>GNVGKISLDQIDLLSTKSFPPCMRQLHKALRENHHLRHGGRMQYGLFLKGIGLTLEQALQFWKQEFIKGKMDPDKFDKGYSYNIRHSFGKEGKRTDYTPFSCLKIILSN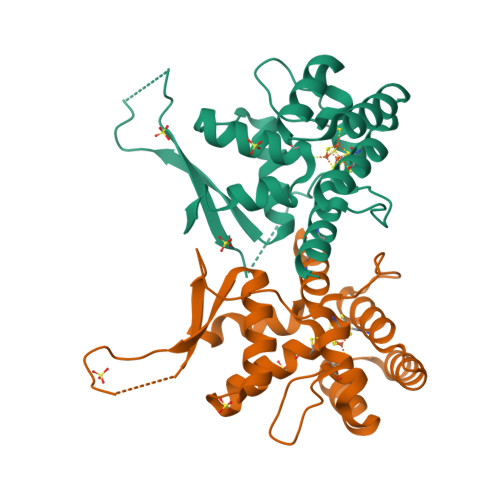PPSQGDYHGCPFRHSDPELLKQKLQSYKISPGGISQILDLVKGTHYQVACQKYFEMIHNVDDCGFSLNHPNQFFCESQRILNG[2x]A chromosome dimer is lethal if unresolved, but most bacteria encode for an efficient site-specific recombination system to convert the chromosome dimers back to monomers, the Xer site-specific recombination system. Most bacteria encode two tyrosine family recombinases XerC and XerD which bind to the specific chromosomal site dif located in the replication terminus region56, although there are notable exceptions where a single Xer protein carries out the reaction. The C-terminal domain of FtsK forms a DNA translocase motor, which also hexamerises, and was found to be essential for chromosome dimer resolution through activation of the XerD recombinase252627. FtsKγ interacts directly with XerD to stimulate its catalytic activity, leading to XerD cutting and exchanging the first pair of strands within a recombinase synapse between dif sites.

To understand how this interaction can lead to activation of recombination, a fusion protein between the C-terminal domain of XerD, which contains the catalytic residues required for DNA cleavage and strand exchange, and FtsKγ was produced (XerDC–γ) and crystallized. The asymmetric unit contained a single XerDC–γ complex, but the flexible linker joining the two protein domains was not visible in the density. The FtsKγ interaction with XerDC is a 563 Å2 interface that involves two helices on the surface of XerDC. These two helices, αE and αH, are on the opposite face from the putative DNA-binding surface of XerD and the active-site residues32. The interaction site on FtsKγ involves the ends of helices α2 and α3 and the loop that joins them3031. It is noteworthy that this is also a region involved in binding of FtsKγ to KOPS DNA, and the amino acids that contact XerD are a subset of those seen to contact DNA; not only is FtsKγ a bi-functional domain with protein-protein and protein-DNA interactions, it uses the same surface to carry out both functions. Although the structure of the fusion protein reveals an interaction surface that is consistent with the proposed role of FtsKγ interacting with and activating XerD whilst it is bound to DNA, there was no obvious structural change in XerD that would account for its activation; the active site residues were in the same, inactive, conformation as seen in the XerD structure without γ present. The E184-R1289 pair interact with each other via a salt bridge and hydrogen bonding in the crystal structure that, based on recombination efficiency, appears to be a critical factor in the interaction.

> MKDLSEAQVERLLQAPLIDQPLELRDKAMLEVLYATGLRVSELVGLTMSDISLRQGVVRVIGKGNKERLVPLGEEAVYWLETYLEHGRPWLLNGVSIDVLFPSQRAQQMTRQTFWHRIKHYAVLAGIDSEKLSPHVLRHAFATHLLNHGADLRVVQMLLGHSDLSTTQIYTHVATERLRQLHQQHHPRAGGGSEGGGSEGGSGSRTGAEELDPLFDQAVQFVTEKRKASISGVQRQFRIGYNRAARIIEQMEAQGIVSEQGHNGNREVLAPPPFD> SSQIRQNYSTEVEAAVNRLV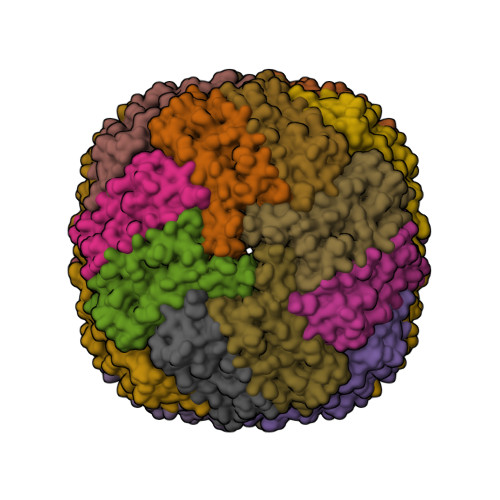NLYLRASYTYLSLGFYFDRDDVALEGVCHFFRELAEEKREGAERLLKMQNQRGGRALFQDLQKPSQDEWGTTLDAMKAAIVLEKSLNQALLDLHALGSAQADPHLCDFLESHFLDEEVKLIKKMGDHLTNIQRLVGSQAGCGEYCFERLTLKHD> MGSSHHHHHHSQDPNSMANPLFRKHIVSINDISRNELELIVKTAAKLKEQPQPELLKNKVIASCFFEASTRT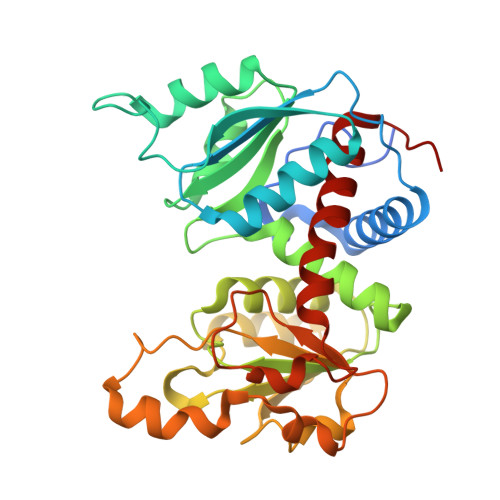RLSFETAIQRLGGSVIGFDNAGNTSLAKKGETLADSISVISSYADAFVMRHPQEGAARLASEFSNVPVINGGDGSNQHPTQTLLDLFSIYETQGRLDNLNIAFVGDLKYGRTVHSLAQALAKFDGCKFHFIAPDALAMPEYICDELDEQNISYATYASIEEVVPEIDVLYMTRVQKERFDETEYQHMKAGFILSASSLVHAKPNLKVLHPLPRVDEIATDVDKTPYAYYFQQAENGVYAREALLALVLNETIGE>MALVLEIFTLLASICWVSANIFEYQVDAQPLRPCELQRETAFLKQADYVPQCAEDGSFQTVQCQNDGRSCWCVGANGSEVLGSRQPGRPVACLSFCQLQKQQILLSGYINSTDTSYLPQCQDSGDYAPVQCDVQQVQCWCVDAEGMEVYGTRQLGRPKRCPRSCEIRNRRLLHGVGDKSPPQCSAEGEFMPVQCKFVNTTDMMIFDLVHSYNRFPDAFVTFSSFQRRFPEVSGYCHCADSQGRELAETGLELLLDEIYDTIFAGLDLPSTFTETTLYRILQRRFLAVQSVISGRFRCPTKCEVERFTATSFGHPYVPSCRRNGDYQAVQCQTEGPCWCVDAQGKEMHGTRQQGEPPSCAEGQSCASERQQALSRLYFGTSGYFSQHDLFSSPEKRWASPRVARFATSCPPTIKELFVDSGLLRPMVEGQSQQFSVSENLLKEAIRAIFPSRGLARLALQFTTNPKRLQQNLFGGKFLVNVGQFNLSGALGTRGTFNFSQFFQQLGLASFLNGGRQEDLAKPLSVGLDSNSSTGTPEAAKKDGTMNKPTVGSFGFEINLQENQNALKFLASLLELPEFLLFLQHAISVPEDVARDLGDVMETVLSSQTCEQTPERLFVPSCTTEGSYEDVQCFSGECWCVNSWGKELPGSRVRGGQPRCPTDCEKQRARMQSLMGSQPAGSTLFVPACTSEGHFLPVQCFNSECYCVDAEGQAIPGTRSAIGKPKKCPTPCQLQSEQAFLRTVQALLSNSSMLPTLSDTYIPQCSTDGQWRQVQCNGPPEQVFELYQRWEAQNKGQDLTPAKLLVKIMSYREAASGNFSLFIQSLYEAGQQDVFPVLSQYPSLQDVPLAALEGKRPQPRENILLEPYLFWQILNGQLSQYPGSYSDFSTPLAHFDLRNCWCVDEAGQELEGMRSEPSKLPTCPGSCEEAKLRVLQFIRETEEIVSASNSSRFPLGESFLVAKGIRLRNEDLGLPPLFPPREAFAEQFLRGSDYAIRLAAQSTLSFYQRRRFSPDDSAGASALLRSGPYMPQCDAFGSWEPVQCHAGTGHCWCVDEKGGFIPGSLTARSLQIPQCPTTCEKSRTSGLLSSWKQARSQENPSPKDLFVPACLETGEYARLQASGAGTWCVDPASGEELRPGSSSSAQCPSLCNVLKSGVLSRRVSPGYVPACRAEDGGFSPVQCDQAQGSCWCVMDSGEEVPGTRVTGGQPACESPRCPLPFNASEVVGGTILCETISGPTGSAMQQCQLLCRQGSWSVFPPGPLICSLESGRWESQLPQPRACQRPQLWQTIQTQGHFQLQLPPGKMCSADYADLLQTFQVFILDELTARGFCQIQVKTFGTLVSIPVCNNSSVQVGCLTRERLGVNVTWKSRLEDIPVASLPDLHDIERALVGKDLLGRFTDLIQSGSFQLHLDSKTFPAETIRFLQGDHFGTSPRTWFGCSEGFYQVLTSEASQDGLGCVKCPEGSYSQDEECIPCPVGFYQEQAGSLACVPCPVGRTTISAGAFSQTHCVTDCQRNEAGLQCDQNGQYRASQKDRGSGKAFCVDGEGRRLPWWETEAPLEDSQCLMMQKFEKVPESKVIFDANAPVAVRSKVPDSEFPVMQCLTDCTEDEACSFFTVSTTEPEISCDFYAWTSDNVACMTSDQKRDALGNSKATSFGSLRCQVKVRSHGQDSPAVYLKKGQGSTTTLQKRFEPTGFQNMLSGLYNPIVFSASGANLTDAHLFCLLACDRDLCCDGFVLTQVQGGAIICGLLSSPSVLLCNVKDWMDPSEAWANATCPGVTYDQESHQVILRLGDQEFIKSLTPLEGTQDTFTNFQQVYLWKDSDMGSRPESMGCRKDTVPRPASPTEAGLTTELFSPVDLNQVIVNGNQSLSSQKHWLFKH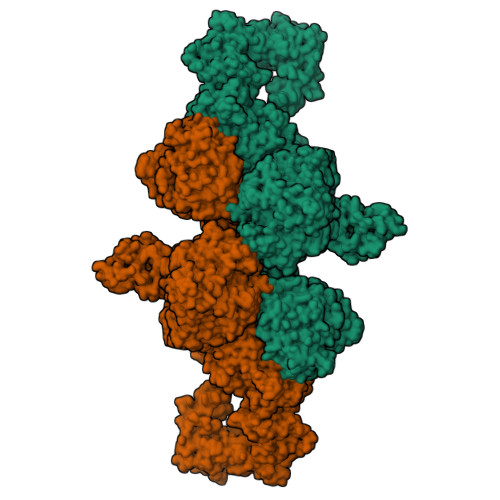LFSAQQANLWCLSRCVQEHSFCQLAEITESASLYFTCTLYPEAQVCDDIMESNAQGCRLILPQMPKALFRKKVILEDKVKNFYTRLPFQKLMGISIRNKVPMSEKSISNGFFECERRCDADPCCTGFGFLNVSQLKGGEVTCLTLNSLGIQMCSEENGGAWRILDCGSPDIEVHTYPFGWYQKPIAQNNAPSFCPLVVLPSLTEKVSLDSWQSLALSSVVVDPSIRHFDVAHVSTAATSNFSAVRDLCLSECSQHEACLITTLQTQPGAVRCMFYADTQSCTHSLQGQNCRLLLREEATHIYRKPGISLLSYEASVPSVPISTHGRLLGRSQAIQVGTSWKQVDQFLGVPYAAPPLAERRFQAPEPLNWTGSWDASKPRASCWQPGTRTSTSPGVSEDCLYLNVFIPQNVAPNASVLVFFHNTMDREESEGWPAIDGSFLAAVGNLIVVTASYRVGVFGFLSSGSGEVSGNWGLLDQVAALTWVQTHIRGFGGDPRRVSLAADRGGADVASIHLLTARATNSQLFRRAVLMGGSALSPAAVISHERAQQQAIALAKEVSCPMSSSQEVVSCLRQKPANVLNDAQTKLLAVSGPFHYWGPVIDGHFLREPPARALKRSLWVEVDLLIGSSQDDGLINRAKAVKQFEESRGRTSSKTAFYQALQNSLGGEDSDARVEAAATWYYSLEHSTDDYASFSRALENATRDYFIICPIIDMASAWAKRARGNVFMYHAPENYGHGSLELLADVQFALGLPFYPAYEGQFSLEEKSLSLKIMQYFSHFIRSGNPNYPYEFSRKVPTFATPWPDFVPRAGGENYKEFSELLPNRQGLKKADCSFWSKYISSLKTSADGAKGGQSAESEEEELTAGSGLREDLLSLQEPGSKTYSK[2x]>HHMSAIKPDMKINLRMEGNVNGHHFVIDGDGTGKPFEGKQSMDLEVKEGGPLPFAFDILTTAFHYGNRVFAEYPDHIQDYFKQSFPKGYSWERSLTFEDGGICIARNDITMEGDTFYNKVRFHGVNFPANGPVMQKKTLKWEPSTEKMYVRDGVLTGDITMALLLEGNAHYRCDSRTTYKAKEKGVKLPGYHLVDHCIEILSHD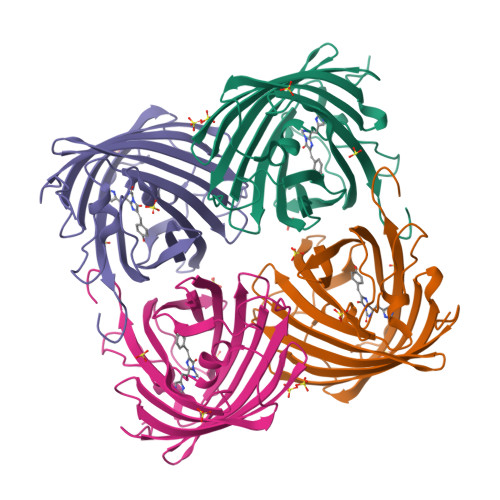KDYNKVKLYEHAVAHSGLPDNARR[4x]> MEAVIFDMDGVLMDTEPLYFEAYRRVAESYGKPYTEDLHRRIMGVPEREGLPILMEALEIKDSLENFKKRVHEEKKRVFSELLK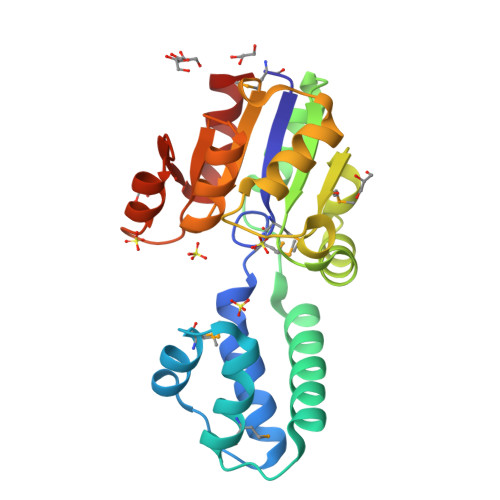ENPGVREALEFVKSKRIKLALATSTPQREALERLRRLDLEKYFDVMVFGDQVKNGKPDPEIYLLVLERLNVVPEKVVVFEDSKSGVEAAKSAGIERIYGVVHSLNDGKALLEAGAVALVKPEEILNVLKEVL> HHHHHHMTTINPTNYTLLKKQAASLIEDEHHMIAILSNMSALLNDNLDQINWVGFYLLEQNELILGP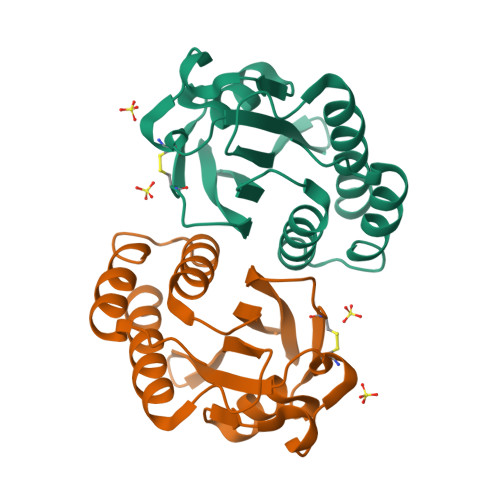FQGHPACVHIPIGKGVCGTAVSERRTQVVADVHQFKGHIACDANSKSEIVVPIFKDDKIIGVLDIDAPITDRFDDNDKEHLEAIVKIIEKQLA> MKLFAQGTSLDLSHPHVMGILNVTPDSFSDGGTHNSLIDAVKHANLMINAGAT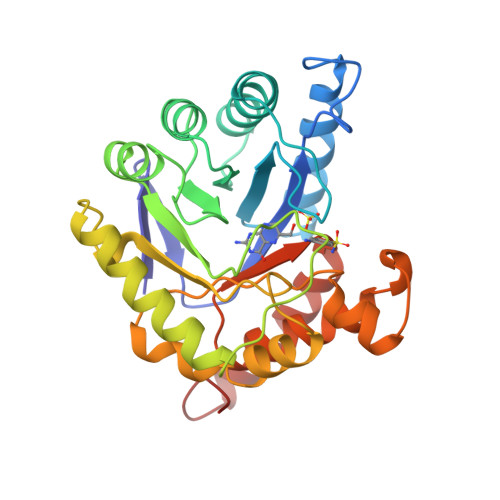IIDVGGESTRPGAAEVSVEEELQRVIPVVEAIAQRFEVWISVDTSKPEVIRESAKVGAHIINDIRSLSEPGALEAAAETGLPVCLMHMQGNPKTMQEAPKYDDVFAEVNRYFIEQIARCEQAGIAKEKLLLDPGFGFGKNLSHNYSLLARLAEFHHFNLPLLVGMSRKSMIGQLLNVGPSERLSGSLACAVIAAMQGAHIIRVHDVKETVEAMRVVEATLSAKENKRYE>SNAMYKEGACLYRNPLRSKSDVKDWRMEGGGQISFDDHSLHLSHVQDEAHFVFWCPETFPDGIIVTWDFSPIEQPGLCMLFFAAAGIRGEDLF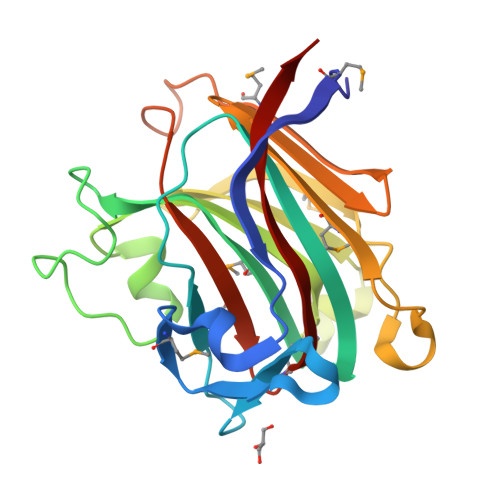DPSLRKRTGTYPEYHSGDINALHLSYFRRKYAEERAFRTCNLRKSRGFHLAAMGADPLPSPDDADSPYRMKLIKDKGYVHFSINGLPILEWMDDGSTYGPVLTKGKIGFRQMAPMKAVYRDFAVHQAVRR[4x]> GAMGSTSLEPTSTLVRVRKSAATLGIAIEGGANTRQPLPRIVTIQRGGSAHNCGQLKVGHVILEVNGQTLRGKEHKEAARIIAEAFKTKERDYI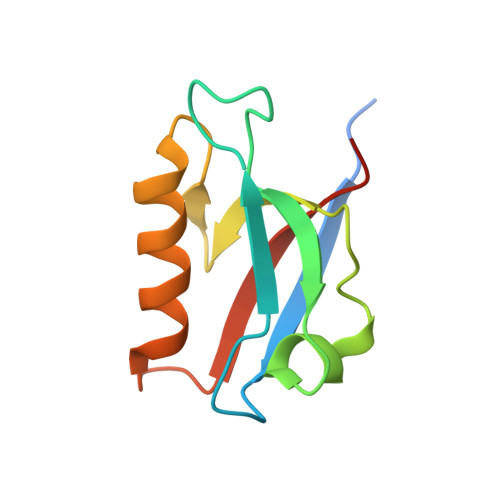DFLVTEFNVML>GPLGSPEPDTARLDADPSASGPVMEFRELQKGAYIEPTGAFLTRARNSVSSSIPYPARAACLLVAVSQATGLPTRTLWAALCANLPDSVLDDGSLATLGLTTDHFAVLARIFSLRCRFVSEHGDVELGLHDATSRFTIRHTPGHFELVADNFSL[2x]

Maize rayado fino virus (MRFV) is the type member of the genus Marafivirus within the family Tymoviridae. The polyprotein characteristically contains four nonstructural domains that comprise the viral replicase (methyltransferase, protease (PRO), helicase (HEL), and RNA-dependent RNA polymerase (RdRp)) as well as the major structural coat protein (CP) for genome packing. The main function of PRO is to act as a polyprotein processor, but it has been shown to have auxiliary function as a ubiquitin (Ub) hydrolase to aid in bypassing the host innate immune system by removing Ub from the RdRp, preventing its degradation by the Ub proteasome. X-ray structures of MRFV PRO alone and bound to Ub reveal unique structural characteristics that differ from TYMV PRO and notable conformational changes that occur in response to Ub substrate.

PRO adopts a compact, three-domain fold, although its C-terminal conformation is held in place by a neighboring copy of the enzyme. The second domain (green panel) is predominantly a well-ordered five-helix bundle (⍺3-⍺7). Helix ⍺3 contains the catalytic cysteine nucleophile (C61) with its solvent-exposed thiol group at the N-terminal end of ⍺3 (Fig. 5A (arrows) and Fig. 5B). Domain III terminates with what appears to be a flexible loop that is solvent exposed until it inserts itself into the active site of a neighboring copy of the enzyme. This loop contains the active site histidine (H144) that is ∼17 Å from the catalytic cystine. The ∼17 Å distance between the side chains of C61 and H144 does not comprise a functional active site. The asymmetric unit (ASU) is composed of two copies of MRFV PRO with most interactions occurring between the alpha helical bundles of domain II of each molecule. The C-terminal tail of each copy of protein in the ASU traverses into its neighbor and appears to complete the active site of the neighboring molecule. The catalytic C61 and incoming His144 residue of the neighboring symmetry mate arrange themselves to within a few angstroms of each other and appear coordinated for catalysis. MRFV PRO is monomeric in solution according to size-exclusion chromatography, and this dimeric interaction between the monomers of the ASU is most likely a crystallographic artifact. Interestingly, aside from the terminal proline (P142), our crystal structure of MRFV PRO reveals that the enzyme lacks a complete GPP motif.>[3x]HEDEIKKLRTSGSMTQNPHEVARVRNLNRIIMGKYEIEPWYFSPYPIELTDEDFIYIDD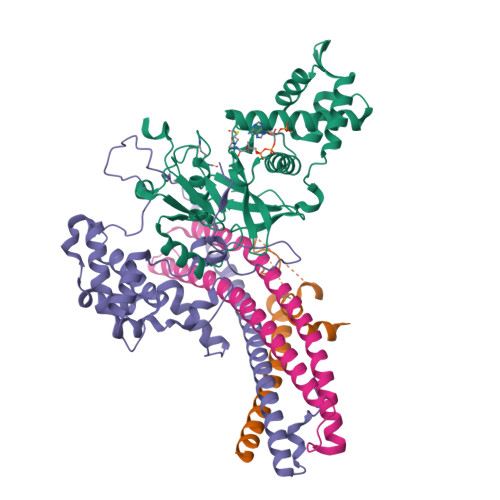FTLQYFGSKKQYERYRKKCTLRHPPGNEIYRDDYVSFFEIDGRKQRTWCRNLCLLSKLFLDHKTLYYDVDPFLFYCMTRRDELGHHLVGYFSKEKESADGYNVACILTLPQYQRMGYGKLLIEFSYELSKKENKVGSPQKPLSDLGLLSYRAYWSDTLITLLVEHQKEITIDEISSMTSMTTTDILHTAKTLNILRYYKGQHIIFLNEDILDRYNRLKAKKRRTIDPNRLIWKPPVFTASQLRFAW;>MTDELKSYEALKAELKKSLQDRREQEDTFDNLQQEIYDKETEYFSHNSNNNHSGHGGAHGSKSHYSGNIIKGFDTFSKSHHSHADSAFNNNDRIFSLSSATYVKQQHGQSQND[3x];>[3x]IPTPDASMTWNEYDKFYTGSFQETTSYIKFSATVEDCCGTNYNMDERDETFLNEQVNKGSSDILTEDEFEILCSSFEHAIHERQPFLSMDPESILSFEELKPTLIKSDMADFNLRNQLNHEINSHKTHFITQFDPVSQMNTRPLIQLIEKFGSKIYDYWRERKIEVNGYEIFPQLKFERPGEKEEIDPYVCFRRREVRHPRKTRRIDILNSQRLRALHQELKNAKDLALLVAKRENVSLNWINDELKIFDQRVKIKNLKRSLNISGEDDDLINHKRKRPT;>MDPSLVLEQTIQDVSNLPSEFRYLLEEIGSNDLKLIEEKKKYEQKESQIHKFIRQQGSIPKHPQEDGLDKEIKESLLKCQSLQREKCVLANTALFLIARHLNKLEKNIALLEEDGVLAPV[3x]quinolin-3-amine | C9 H8 N2 | 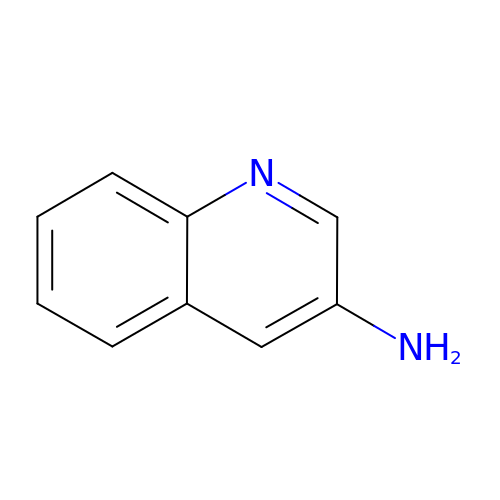SVNCRRZKBNSMIV-UHFFFAOYSA-N>MDKTISVIGMPMDLGQARRGVDMGPSAIRYAHLIERLSDMGYTVEDLGDIPINREKIKNDEELKNLNSVLAGNEKLAQKVNKVIEEKKFPLVLGGDHSIAIGTLAGTAKHYDNLGVIWYDAHGDLNTLETSPSGNIHGMPLAVSLGIGHESLVNLEGYAPKIKPENVVIIGARSLDEGERKYIKESGMKVYTMHEIDRLGMTKVIEETLDYLSACDGVHLSLDLDGLDPNDAPGVGTPVVGGISYRESHLAMEMLYDAGIITSAEFVEVNPILDHKNKTGKTAVEL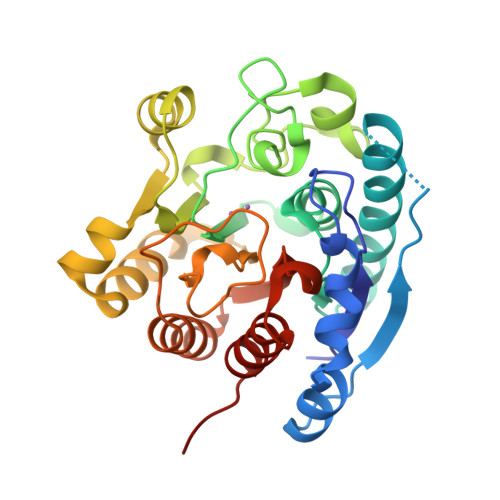VESLLGKKLL[6x]FKBP12 proteins are members of the FKBP PPIase (peptidyl-prolyl isomerase) superfamily and catalyze the cis-trans isomerization of proline imidic peptide bonds. The immunosuppressants first bind to their respective immunophilins, FKBP12 (12-kDa FK506 binding protein) and CypA (cyclophilin A), which subsequently bind to calcineurin in a groove between the CnA and CnB subunits. The immunophilin-immunosuppressant complexes inhibit calcineurin serine-threonine phosphatase activity, blocking the dephosphorylation of downstream targets, such as the human nuclear transcription factor NFAT (nuclear factor of activated T cells), involved in T-cell activation and interleukin-2 transcription, and the fungal transcription factor Crz1 (NFAT homolog), implicated in virulence, stress response, and thermotolerance. To this end, we characterized high-resolution structures of the Mucor circinelloides FKBP12 bound to FK506 and of the Aspergillus fumigatus, M. circinelloides, and human FKBP12 proteins bound to the FK506 analog APX879, which exhibits enhanced selectivity for fungal pathogens.

The FK506 analog APX879, substituted on the C22-ketone with an acetohydrazine moiety, was hypothesized, based on our structural data, to introduce a steric clash with hFKBP12-His88, potentially benefiting fungal selectivity. Crystals of hFKBP12, AfFKBP12, and McFKBP12 bound to APX879 diffracted at resolutions of 1.7, 1.6, and 1.9 Å, respectively. The FKBP12-APX879 structures showed minimal structural variations compared to their FK506-bound counterparts (Cα-RMSDs, ∼0.5 Å), maintaining similar H-bond patterns (i.e., 4 to 5): two with the backbone of residues Gluh/ArgAf/GlnMc55 and Ile57 and two or three with the side chain of residues Tyr27, Asp38, and Tyr83. Interestingly, when bound to McFKBP12, the APX879 acetohydrazine moiety adopts a third conformation with a C21-C22 dihedral angle of −92° leading to a ∼130° flip compared to FK506-C22 ketone (McFKBP12-FK506 C21-C22 dihedral angle, ∼32°). The adoption of this conformation prevents steric clashes with McFKBP12-Tyr88, positioned ∼3 Å away from APX879-C60 when overlaid with McFKBP12-FK506. Altogether, the crystal structures suggest that the flexibility of the acetohydrazine moiety compensates, at least in part, for the bulkiness of the amino acids at position 88. The affinity for APX879 was reduced by ∼40-fold for hFKBP12 and McFKBP12 (KD, ∼120 nM) and 100-fold for AfFKBP12 (KD = 462 ± 23 nM). McFKBP12 also showed peak doubling, not seen when bound to FK506, for an increased number of residues located in the 40’s, 50’s, and 80’s loop (Ser39, Arg41, Arg43, Arg48 to -50, Arg52 to -53, Arg56 to -60, Arg83 to -84, Arg86, Tyr88, Leu91, and Glu103) when bound to APX879, while no peak doubling was observed for AfFKBP12 when bound to either ligand.

> GSHMGVTVERIAPGDGKNFPKKGDKVTIHYVGTLENGDKFDSSRDRGSPFQCTIGVGQVIKGWDEGVTQLSVGEKARLICTHDYAYGERGYPGLIPPKATLNFEVELIKIN>[4x]MSQHNEKNPHQHQSPLHDSSEAKPGMDSLAPEDGSHRPAAEPTPPGAQPTAPGSLKAPDTRNEKLNSLEDVRKGSENYALTTNQGVRIADDQNSLRAGSRGPTLLEDFILREKITHFDHERIPERIV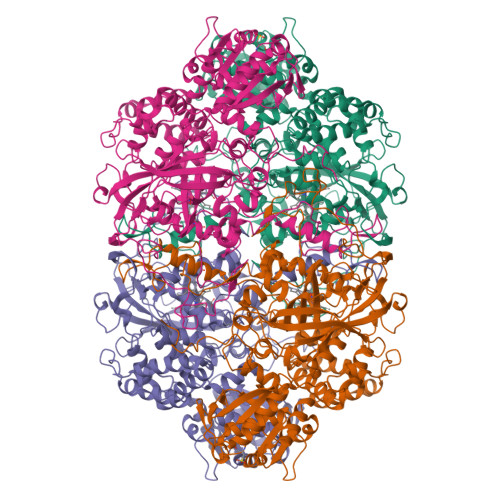HARGSAAHGYFQPYKSLSDITKADFLSDPNKITPVFVRFSTVQGGAGSADTVRDIRGFATKFYTEEGIFDLVGNNTPIFFIQDAHKFPDFVHAVKPEPHWAIPQGQSAHDTFWDYVSLQPETLHNVMWAMSDRGIPRSYRTMEGFGIHTFRLINAEGKATFVRFHWKPLAGKASLVWDEAQKLTGRDPDFHRRELWEAIEAGDFPEYELGFQLIPEEDEFKFDFDLLDPTKLIPEELVPVQRVGKMVLNRNPDNFFAENEQAAFHPGHIVPGLDFTNDPLLQGRLFSYTDTQISRLGGPNFHEIPINRPTCPYHNFQRDGMHRMGIDTNPANYEPNSINDNWPRETPPGPKRGGFESYQERVEGNKVRERSPSFGEYYSHPRLFWLSQTPFEQRHIVDGFSFILSKVVRPYIRERVVDQLAHIDLTLAQAVAKNLGIELTDDQLNITPPPDVNGLKKDPSLSLYAIPDGDVKGRVVAILLNDEVRSADLLAILKALKAKGVHAKLLYSRMGEVTADDGTVLPIAATFAGAPSLTVDAVIVPCGNIADIADNGDANYYLMEAYKHLKPIALAGDARKFKATIKIADQGEEGIVEADSADGSFMDELLTLMAAHRVWSRIPKIDKIPA>RPSGRKSSKMQAFRIWDVNQKTFYLRNNQLVAGYLQGPNVNLEEKIDVVPIEPHALFLGIHGGKMCLSCVKSGDETRLQLEAVNITDLSENR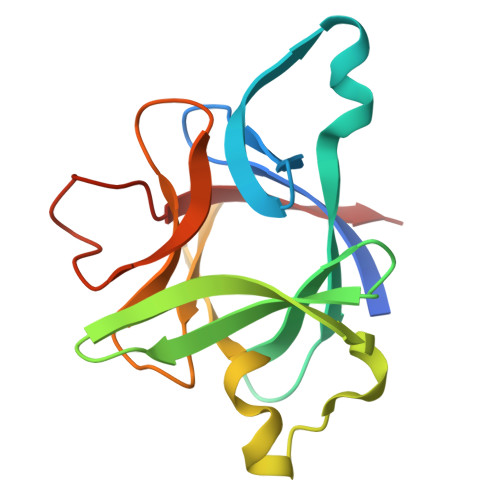KQDKRFAFIRSDSGPTTSFESAACPGWFLCTAMEADQPVSLTNMPDEGVMVTKFYFQEDE[2x]>[2x]ITGQAACPESWIGFQRKCFYFSDDTKNWTSSQRFCDSQDADLAQVESFQELNFLLRYKGPSDHWIGLSREQGQPWKWINGTEWTRQFPILGAGECAYLNDKGASSARCYTERKWICSKSDIHVGTKHHHHHHHHG;>[4x]ETGGLLNCPIYWQQLREKCLLFSHTVNPWNNSLADCSTKESSLLLIRDKDELIHTQNLIRDKAILFWIGLNFSLSEKNWKWINGSFLNSNDLEIRGDAKENSCISISQTSVYSEYCSTEIRWICQKELTPVRNKVYPDSKHHHHHH

Signaling by the human C-type lectin-like receptor, natural killer (NK) cell inhibitory receptor NKR-P1, has a critical role in many immune-related diseases and cancer. Human NKR-P1 and LLT1 are type II transmembrane glycoproteins with similar protein topology: an N-terminal cytoplasmic signaling tail, a transmembrane helix, a flexible stalk region, and a C-terminal C-type lectin-like domain (CTLD). In addition, NKR-P1 promotes transendothelial migration to immunologically privileged niches upon interaction with its endogenous ligand, lectin-like transcript 1 (LLT1). Here we report the crystal structures of the NKR-P1 and NKR-P1:LLT1 complexes, which provides evidence that NKR-P1 forms homodimers in an unexpected arrangement to enable LLT1 binding in two modes, bridging two LLT1 molecules.

The crystal structure of the NKR-P1:LLT1 complex is formed by deglycosylated NKR-P1 and LLT1 ectodomains. The asymmetric unit of the crystal contains a complex of dimeric NKR-P1 with dimeric LLT1 and an extra dimer of NKR-P1. These NKR-P1 dimers have the same helix α1-centered dimerization interface as the structures of the unbound NKR-P1 dimers described above. The LLT1 homodimer engages its partner bivalently, i.e., one dimer interacts with two NKR-P1 dimers related by crystallographic symmetry: each LLT1 monomer binds to a different subunit of a distinct NKR-P1 homodimer. NKR-P1 and LLT1 establish two types of contact in this structure – the primary (LLT1 chain B:NKR-P1 chain D) and the secondary (LLT1 chain A:NKR-P1 symmetry-related chain C) interaction modes. The primary interaction mode is established through nine direct and several water-mediated hydrogen bonds, in addition to two charge-supported and π-π stacking (Tyr201-Arg175) interactions, with a total contact surface area of ca. 800 Å2. The second interaction mode is established through five direct hydrogen bonds, two charge-supported and a hydrophobic (LLT1:Pro156 – NKR-P1:Ala149, Leu151) interaction, with a total contact surface area of ca. 550 Å2. Besides interaction with LLT1, NKR-P1 dimers bound in primary and secondary modes also have non-negligible mutual accessory contact (NKR-P1 chain D and NKR-P1 chain C in symmetry-related position, Csym). Interestingly, in the present structure of this complex, we indeed observe the formation of a chain of repeating NKR-P1 and LLT1 homodimers. This pseudo-linear multimer has a zigzag shape in which the membrane-proximal parts of the two proteins are on opposite sides, and it is structurally based on the alternating helix α1/α2-centered NKR-P1/LLT1 homodimers (the chain-forming effect) and the simultaneous involvement of both primary and secondary interaction modes (steric effect).> GSLHESPYADPEEIRPKEVYLDRKLLTLEDKELGSGNFGTVKKGYYQMKKVVKTVAVKILKNEANDPALKDELLAEANVMQQLDNPYIVRMIGICEAESWMLVMEMAELGPLNKYLQQNRHVKDKNIIELVHQVSMGMKYLEESNFVHRDLAARNVLLVTQHYAKISDFGLSKALRADENY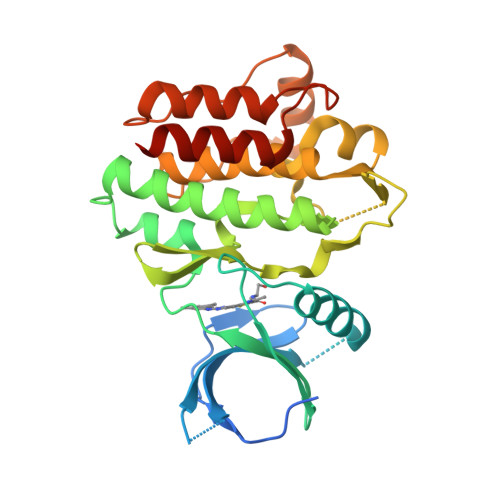YKAQTHGKWPVKWYAPECINYYKFSSKSDVWSFGVLMWEAFSYGQKPYRGMKGSEVTAMLEKGERMGCPAGCPREMYDLMNLCWTYDVENRPGFAAVELRLRNYYYDVVN>ATAAEIAALPRQKVELVDPPFVHAHSQVAEGGPKVVEFTMVIEEKKIVIDDAGTEVHAMAFNGTVPGPLMVVHQDDYLELTLINPETNTLMHNINFHAATGALGGGGLTEINPGEKTILRFKATKPGVFVYHCAPPGMVPWHVVSGMNGAIMVLPREGLHDGKGKALTYDKIYYVGEQDFYVPRDENGKYKKYEAPGDAYEDTVKVMRTLTPTHVVFNGAVGALTGDKAMTAAVGEKVLIVHSQANRDTRPHLIGGHGDYVWATGKFNTPPDVDQETWFIPGGAAGAAFYTFQQPGIYAYVNHNLIEAFELGAAAHFKVTGEWNDDLM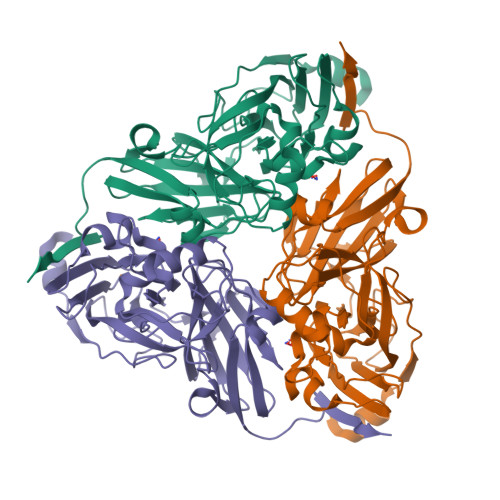TSVLAPSGTIEGR[3x]The dipeptidyl peptidases (DPP) 8 and 9 are serine proteases of the dipeptidyl peptidase 4 activity/structure homologues (DASH) subfamily which cleave post-proline bonds two residues from the N-terminus of a substrate. While DPP4 and FAP are extracellular or secreted proteases, DPP8 and DPP9 are located intracellularly to the cytoplasm and nucleus. There, they play important roles in diverse biological processes such as pyroptosis or ubiquitin-mediated proteolysis, turning them into promising targets for chemical probe and anti-inflammatory or anticancer drug discovery. Here, we show the exploration of the natural product Sulphostin, a DPP4 inhibitor, as a starting point for DPP8/9 inhibitor development.

To verify that the synthesized derivatives share the same binding mode as the parent compound Sulphostin and to elucidate the structural basis of their inhibition potency, a crystal structure of the most potent N-phosphono-(S)-3-aminopiperidine-2-one, compound 16, and DPP9 was analyzed. Analogous to Sulphostin, the electron density revealed a covalent modification of the catalytically active serine residue (S730) of DPP9, this time with a corresponding 2-(4-pentylphenylthio)ethylphosphonate moiety, confirming that the (S)-3-aminopiperidine-2-one moiety also here acts as a leaving group. Although an epimeric mixture of (3S, RP) and (3S, SP) diastereomers of 16 was added, the electron density showed that the phosphorus atom is exclusively in an SP configuration after nucleophilic attack by the active site serine, indicating that the active diastereomer has the (3S, RP)-configuration, again matching with the spatial arrangement found in Sulphostin. The ethoxy group of the phosphonate binds to the hydrophobic S1 sub-site formed by V756, V811 and Y762. The 2-(4-pentylphenylthio)ethyl residue extends towards the S’ region and then bends sharply to protrude into the S2 pocket. Specifically, the pentyl tail occupies the S2 pocket, however, it appears highly flexible due to the lack of strong specific interactions with the protein. The whole binding mode is further stabilized by a specific hydrogen bond between the phosphoryl oxygen and the Y644 side chain. In an attempt to combine the inhibition features of the aromatic system with the observed improved inhibition of longer alkyl chains, compound 16 was synthesized and showed the strongest inhibition of DPP8 with an IC50 of 14 ± 1 nM and best selectivity over DPP9 ( ~21-fold) and DPP4 ( ~1154-fold) of all tested derivatives. The rate constants for irreversible inactivation were consistent with IC50 values, proving the high potency and selectivity of 16, as a kapp of 20 M−1 s−1 was determined for DPP4, 51,249 M−1 s−1 for DPP8 and 2310 M−1 s−1 for DPP9.

>[4x]MPAARFQVQKHSWDGLRSIIHGSRKYSGLIVNKAPHDFQFVQKTDESGPHSHRLYYLGMPYGSRENSLLYSEIPKKVRKEALLLLSWKQMLDHFQATPHHGVYSREEELLRERKRLGVFGITSYDFHSESGLFLFQASNSLFHCRDGGKNGFMVSPMKPLEIKTQCSGPRMDPKICPADPAFFSFINNSDLWVANIETGEERRLTFCHQGLSNVLDDPKSAGVATFVIQEEFDRFTGYWWCPTASWEGSEGLKTLRILYEEVDESEVEVIHVPSPALEERKTDSYRYPRTGSKNPKIALKLAEFQTDSQGKIVSTQEKELVQPFSSLFPKVEYIARAGWTRDGKYAWAMFLDRPQQWLQLVLLPPALFIPSTENEEQRLASARAVPRNVQPYVVYEEVTNVWINVHDIFYPFPQSEGEDELCFLRANECKTGFCHLYKVTAVLKSQGYDWSEPFSPGEDEFKCPIKEEIALTSGEWEVLARHGSKIWVNEETKLVYFQGTKDTPLEHHLYVVSYEAAGEIVRLTTPGFSHSCSMSQNFDMFVSHYSSVSTPPCVHVYKLSGPDDDPLHKQPRFWASMMEAASCPPDYVPPEIFHFHTRSDVRLYGMIYKPHALQPGKKHPTVLFVYGGPQVQLVNNSFKGIKYLRLNTLASLGYAVVVIDGRGSCQRGLRFEGALKNQMGQVEIEDQVEGLQFVAEKYGFIDLSRVAIHGWSYGGFLSLMGLIHKPQVFKVAIAGAPVTVWMAYDTGYTERYMDVPENNQHGYEAGSVALHVEKLPNEPNRLLILHGFLDENVHFFHTNFLVSQLIRAGKPYQLQIYPNERHSIRCPESGEHYEVTLLHFLQEYLHHHHHH>[2x]GPGGTMGRVTAPEPLSAFHQVAEFVSGEAVLDDWLKQKGLKNQALGAARTFVVCKKDTKQVAGFYSLATGSVNHTEATGNLRRNMPDPIPVIILARLA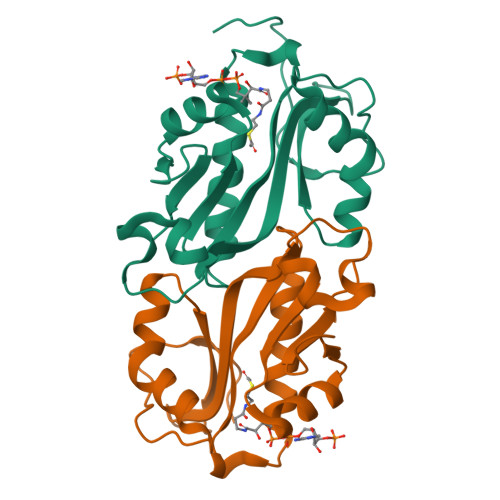VDLSFHGKGLGADLLHDAVLRCYRVAENIGVRAIMVHALTEEAKNFFIHHGFKSSQTQQRTLFLRLPQ>[6x]MAHHHHHHMADGDDTALTNLVALASQRLALAEPVAHWKWINRKPI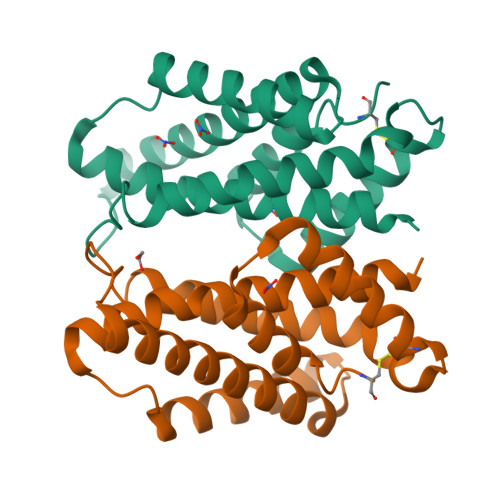SDPPREAALLTDVEKRATANGVDPAYARTFFDDQIAASKQLQNALFATWRATHGPEGPAPDLATSTRPQLDRLTQSLIAALARVAPLRDAPDCPSRLARSIANWKTLTRYDSAQKDALGTALSHVCAAGGASAVG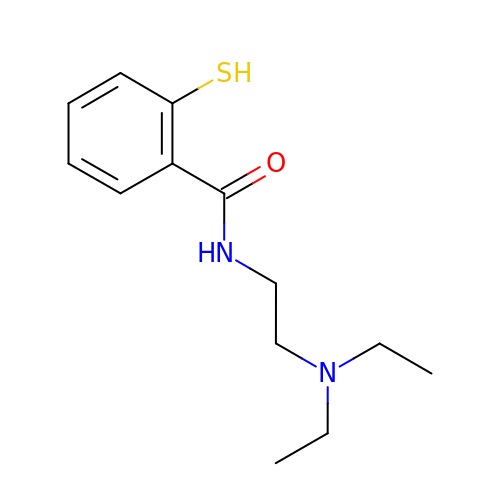~{N}-[2-(diethylamino)ethyl]-2-sulfanyl-benzamide | C13 H20 N2 O S | MFTVFFIYFANPCV-UHFFFAOYSA-N>GSMETSMPEYYEVFGEFRGVLMDKRFTKYWEDVEMFLARPDDLVIATYPKSGTTWISEVVYMIYKEGDVEKCKEDAIFNRIPYLECRNEDLINGIKQLKEKESPRIVKTHLPPKLLPASFWEKNCKMIYLCRNAKDVAVSYYYFLLMITSYPNPKSFSEFVEKFMQGQVPYGSWYDHVKAWWEKSKNSRVLFMFYEDMKEDIRREVVKLIEFLERKPSAELVDRIIQHTSFQEMKNNPSTNYTMMPEEMMNQKVSPFMRKGIIGDWKNHFPEALRERFDEHYKQQMKDCTVKFRM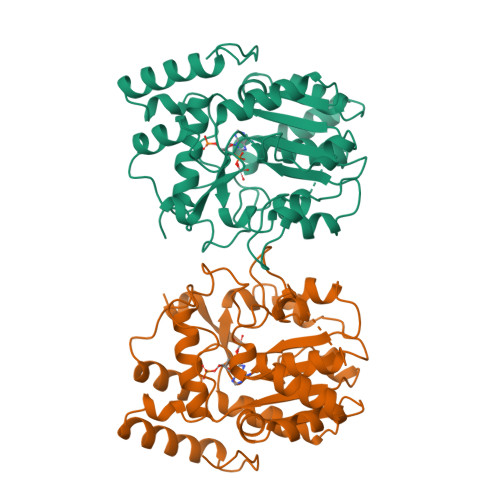EL[2x]3-[2-[(Z)-[5-[(Z)-[(3R,4R)-3-ethenyl-4-methyl-5-oxidanylidene-pyrrolidin-2-ylidene]methyl]-3-(3-hydroxy-3-oxopropyl)-4-methyl-pyrrol-2-ylidene]methyl]-5-[(Z)-(4-ethenyl-3-methyl-5-oxidanylidene-pyrrol-2-ylidene)methyl]-4-methyl-1H-pyrrol-3-yl]propanoic 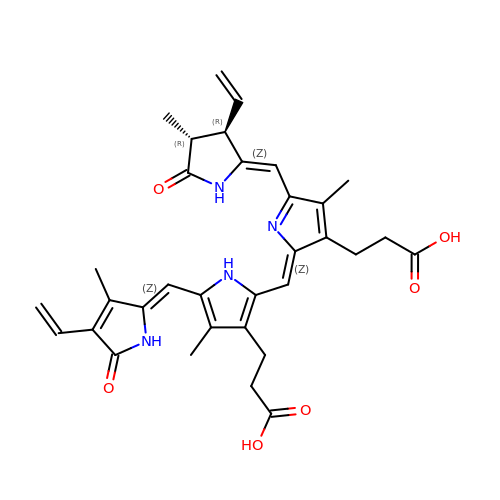acid | C33 H36 N4 O6 | WLDQKQLRZDEERT-IFTFHFPBSA-N In addition to transcripts encoding an FP clearly homologous to A. victoria green fluorescent protein (avGFP), as we expected, the A. cf. australis transcriptome also contains several transcripts encoding other, much more divergent avGFP homologs. Characterization of the recombinant proteins revealed that these avGFP homologs include a green-emitting FP that appears to be the brightest FP discovered to date, 2 long-wavelength-absorbing CPs, and a reversibly photochromic FP (Figs 1Β and 2). We have identified several new Aequorea FPs with the potential to further diversify the landscape of fluorescent probes and biosensors.

AausFP2 has a distinctive cyan-blue pigmented appearance when expressed in E. coli, with a broad absorbance spectrum peaking at 610 nm. Every Aequorea CP displays a broad absorbance spectrum that lacks the well-defined sharp peak and short-wavelength shoulder typical of most FPs and CPs, suggesting that these proteins contain an unusual chromophore and/or chromophore environment. X-ray crystallography analysis of AausFP2 revealed a conserved dimer interface geometry containing many conserved residues between AausFP1 and AausFP2. We suspect that despite AausFP2’s behavior in gel filtration experiments, the native oligomeric state of AausFP2 may be a dimer. The amino acid residues making up the dimer interface in the AausFP2 crystal structure are also largely conserved across the other Aequorea CPs, suggesting that if this is the native oligomeric state of AausFP2, then they are all likely to be dimers. The X-ray crystal structure of AausFP2 further revealed a chemically novel chromophore in which the side chain of a neighboring cysteine is covalently linked to the methylene bridge of a twisted GFP-like chromophore. This amino acid, Cys62, is conserved in all Aequorea CPs. The C62S mutant of AausFP2 appears yellow and has a major absorbance peak characteristic of a GFP-type chromophore, strongly suggesting that this conserved cysteine is necessary for formation of the red-shifted chromophore. Quantum mechanical calculations indicate that both the presence of a sulfur atom and a twisted chromophore are required to produce long-wavelength absorbance. Because of its broad absorbance reaching into the far-red and near-infrared regions of the spectrum, its relatively high extinction coefficient, and its efficient folding at 37°C, AausFP2 or its derivatives could ultimately prove very useful as photoacoustic tomography probes for deep tissue imaging.

> MACGALLFKGKIPFVVELEGDVNGEVFSVRGNGWGDGSTGKLEIKFVCTTGEVPLAWESLICSMAYGALVFCKYPSNINDFFKSTMPRGYIQERKISYENDGTFDVRQEVTYENGALYNRVKFNGSGFRKDGNVLGKKLDLTSIGTCIYIMGNDEGTGLKGVFNKAFKVIGGNRQIASHVQTQTPIGDGLVSIPDYHVMHNHIACSKDPSETRDHIIVKESLRAVDCNTEYM> DRVYIHPFHLVIHNESTCEQLAKANAGKPKDPTFIPAPIQAKTSPVDEKALQDQLVLVAAKLDTEDKLRAAMVGMLANFLGFRIYGMHSELWGVVHGATVLSPTAVFGTLASLYLGALDHTADRLQAILGVPWKDKQCTSRLDAHKVLSALQAVQGLLVAQGRADSQAQLLLSTVVGVFTAPGLHLKQPFVQGLALYTPVVLPRSLDFTELDVAAEKIDRFMQAVTGWKTGSSLMGASVDSTLAFNTYVHFQGKMKGFSLLAEPQEFWVDQSTSVSVPMLSGMGTFQHWSDIQDQFSVTQVPFTESASLLLIQPHYASDLDKVEGLTFQQNSLNWMKKLSPRTIHLTMPQLVLQGSYDLQDLLAQAELPAILHTELNLQKLSNDRIRVGEVLNSIFFELEADEREPTESTQQLNKPEVLEVTLNRPFLFAVYDQSATALHFLGRVANPLSTAHH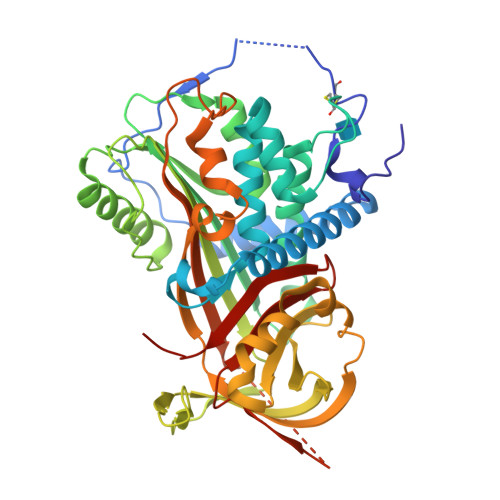HHHH(1~{R},2~{S},3~{R},4~{R},5~{S},6~{R})-5-azanyl-6-(hydroxymethyl)cyclohexane-1,2,3,4-tetrol | C7 H15 N O5 | 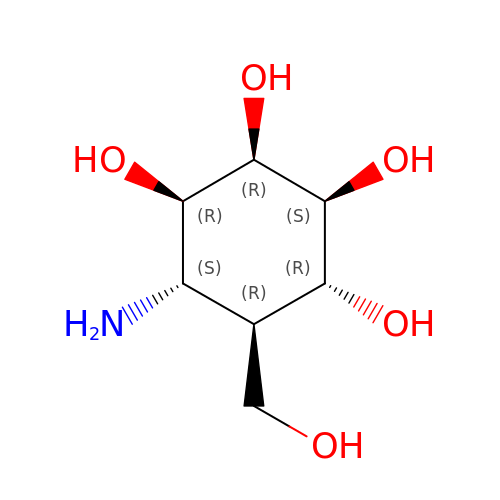SWVTZDDSAFUTKS-BJUQCWQQSA-N(2S)-3-hydroxypropane-1,2-diyl ditetradecanoate | 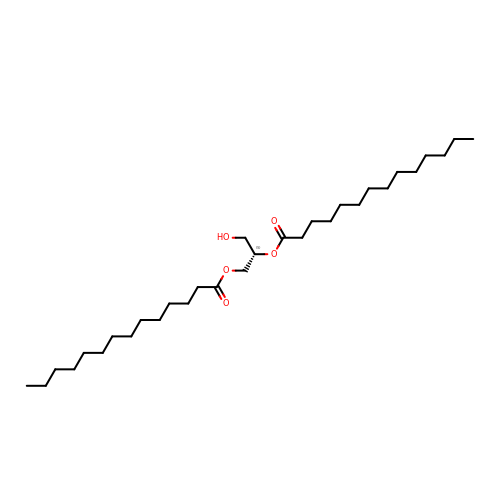C31 H60 O5 | JFBCSFJKETUREV-LJAQVGFWSA-N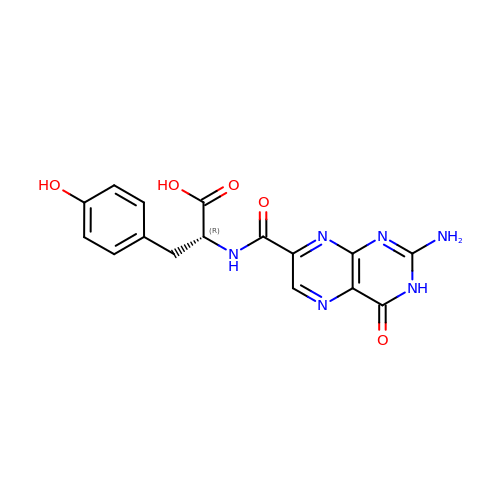(2R)-2-[(2-azanyl-4-oxidanylidene-3H-pteridin-7-yl)carbonylamino]-3-(4-hydroxyphenyl)propanoic acid | C16 H14 N6 O5 | BYYDVPCOJAQWPZ-SECBINFHSA-N>DSRGCARWCPQDSSCVNATACRCNPGFSSFSEI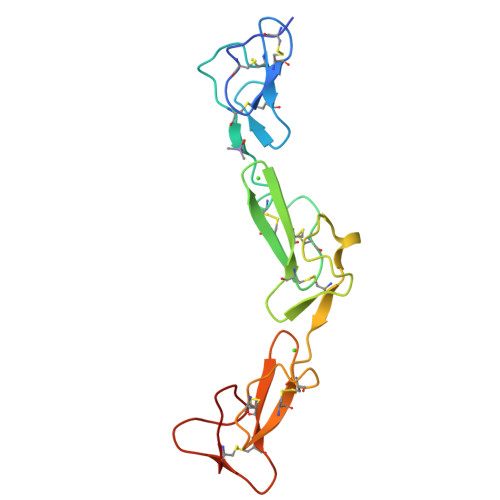ITTPMETCDDINECATLSKVSCGKFSDCWNTEGSYDCVCSPGYEPVSGAKTFKNESENTCQDVDECSSGQHQCDSSTVCFNTVGSYSCRCRPGWKPRHGIPNNQKDTVCE[2x]>[2x]GMRPALYFCGSIRGGREDRTLYERIVSRLRRFGTVLTEHVAAAELGARGEEAAGGDRLIHEQDLEWLQQ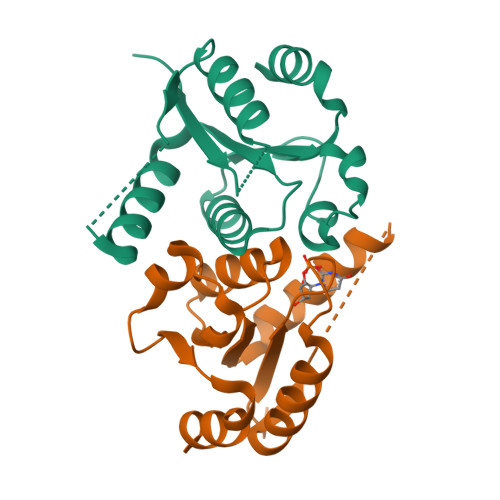ADVVVAEVTQPSLGVGYELGRAVAFNKRILCLFRPQSGRVLSAMIRGAADGSRFQVWDYEEGEVEALLDRYFEADP> GMDYNQTVLSHLQKFWKHHDIKGFTWTLGRIVEELPDFQVFQVIPNHEDEPWVYVSSGIGQFLGQEFFIISPFETPEHIET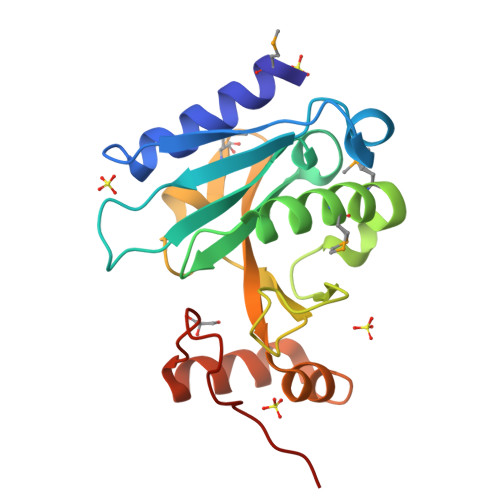LAMLASASMHYPDQFQLGKTVNIGRPWVEQSSFRHFLISLPYPYGQELEYMDNVRFFWLLPITQTERLFLNTHSVEELETKFDEAGIDYLDINRASTVWQAG>MPKPYVAINMVEVRNDPKTLELFGKVGPKVCMVTARHPGFVGFQNHVQIGVVPLGTRWGGAKMEMSQEMHSLMLMQYTFWKNWKDHEEMHKQNWANLFRLCLQCADQMIWGPYEPLYEIVYANMPLNTEMTDFTVMVGKKFAAGEAVSIPPISQPYGKRVVAFGEHIVKEGLENQFEEYAIKTLEAFRSAPGFLGGMILKEIGVSPLGSLQLNAKGFHQILETANGMDVPEPVTIYEAPEFRNRPQRYIVHTEWSDTNALMFGLGRVLIYPEVRQIHDKVLDTLVYGPYIRVLNPMMEGTYWREYLNEYHL[24x]

Sulfur oxygenase reductases (SORs) are present in thermophilic and mesophilic archaea and bacteria, and catalyze oxygen-dependent oxygenation and disproportionation of elemental sulfur. SOR has a hollow, spherical homo-24-mer structure and reactions take place at active sites inside the chamber. Here, we report the biochemical and structural characterizations of SORs from the thermoacidophilic archaeon Sulfurisphaera tokodaii (StSOR) and present high-resolution structures determined by X-ray crystallography and cryogenic electron microscopy (cryo-EM). Each monomer has an 8-stranded β barrel core surrounded by 10 α helices.

The cryo-EM structure was determined at 2.24 Å resolution using an instrument operating at 200 kV. The cryo-EM analysis was conducted with octahedral symmetry from ab initio 3D reconstruction to the final 3D refinement and model reconstruction. The reconstructed cryo-EM structure consisted of 24 identical polypeptides with residues from Pro2 to Leu311. The overall cryo-EM structure of StSOR was almost the same as determined by the crystal structure. The ligands were similarly located as those of the crystal structure, except that Wat2 was not observed. The CheckMyMetal server indicated trigonal bipyramidal 5-coordination with an outlier nVECSUM of 0.26 and the distances between the iron atom and the ligands were slightly greater than those in the crystal structure. The cryo-EM maps around Cys31 and Cys104 exhibited different features compared with the crystal structure, while Cys101 was also observed as a non-flexible free thiol. The map around Cys31 is extended with a branch. The lengths of the extensions toward the iron and Cys104 are ~4.0 Å and ~3.4 Å, respectively at a 0.0435 (4.5σ) contour level. These lengths correspond to approximately two disulfide bonds (2.05 Å for each), thus implying formation of a persulfide, trisulfide, or branched oligosulfides. On the other hand, chimneys were determined with lower local resolution than inside the molecule in the cryo-EM structure, and the map of the side chains are more ambiguous.XIAP (X-linked inhibitor of apoptosis) directly inhibits the upstream caspase-9 and the downstream caspase-3 and caspase-7, and therefore controls critical apoptotic checkpoints. The XIAP protein consists of several domains, including three zinc-containing BIR (baculovirus IAP repeat) domains (BIR1, BIR2 and BIR3) and a C-terminal RING domain. The linker region blocks the active sites of these caspases, while the N-terminal regions of the partially processed caspase-3 and caspase-7 bind the BIR2 domain in a peptide-binding groove that accommodates the four N-­terminal residues. As has been reported previously for other BIR domains, the overall architecture of the BIR2 domain is a three-stranded antiparallel β-sheet surrounded by five α-helices, with a structurally important zinc residue coordinated by Cys200, Cys203, His220 and Cys227.

Smac also binds in the same groove of XIAP through its N-terminal IAP-binding motif, AVPI, and associates primarily with the BIR3 domain, although it also has affinity for the BIR2 domain. Therefore, the structures of XIAP BIR2 with five different peptides soaked in and bound to the Smac binding groove were also solved: ATAA, AVPI, SVPI, AIAV and AMRV. The additional hydroxyl introduced by the serine substitution results in only a small shift in the side chains of His223 and Leu207 to allow the extra atom. We have shown in a series of peptide-bound structures that the protein is somewhat flexible and can adjust the conformation of the side chains in the binding groove to accommodate differences in the peptide.

>GTIYPRNPAMYSEEARLKSFQNWPDYAHLTPRELASAGLYYTGIGDQVQCFACGGKLKNWEPGDRAWSEHRRHFPNCFFVLGRNLN[2x];> AVPI>GPAESLPDLKIEKLDEGVYVHTSFEEVNGWGVVPKHGLVVLVNAEAYLIDTPFTAKDTEKLVTWFVERGYKIKGSISSHFHSDSTGGIEWLNSRSIPTYASELTNELLKKDGKVQATNSFSGVNYWLVKNKIEVFYPGPGHTPDNVVVWLPERKILFGGCFIKPYGLGNLGDANIEAWPKSAKLLKSK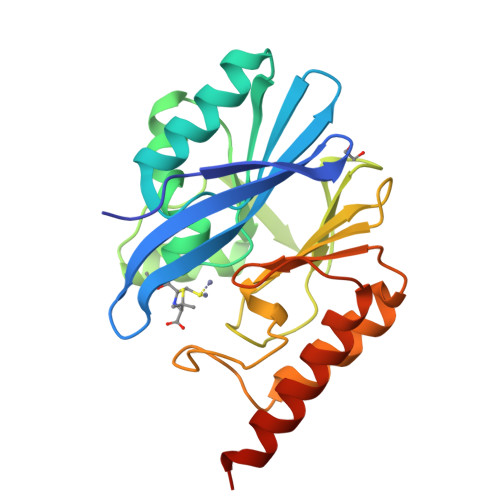YGKAKLVVPSHSEVGDASLLKLTLEQAVKGLNESKKPSKPSN[4x]> GP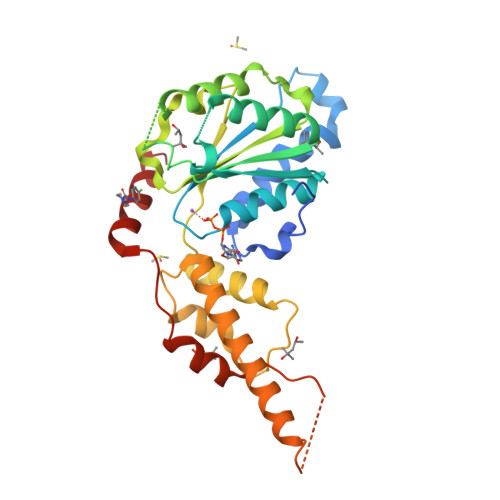GSALRETVVEVPQVTWEDIGGLEDVKRELQELVQYPVEHPDKFLKFGMTPSKGVLFYGPPGCGKTLLAKAIANECQANFISIKGPELLTMWFGESEANVREIFDKARQAAPCVLFFDELDSIAKARGGNIGDGGGAADRVINQILTEMDGMSTKKNVFIIGATNRPDIIDPAILRPGRLDQLIYIPLPDEKSRVAILKANLRKSPVAKDVDLEFLAKMTNGFSGADLTEICQRACKLAIRESIESEIRRERERQTNPSAMEVEEDDPVPEIRRDHFEEAMRFARRSVSDNDIRKYEMFAQTLQQ> MITENEKISLPKIDWALDALEPYISKEINDLHINKHHVAYVNGYNAAIDALEKAVGKRDLKSVVEIQQ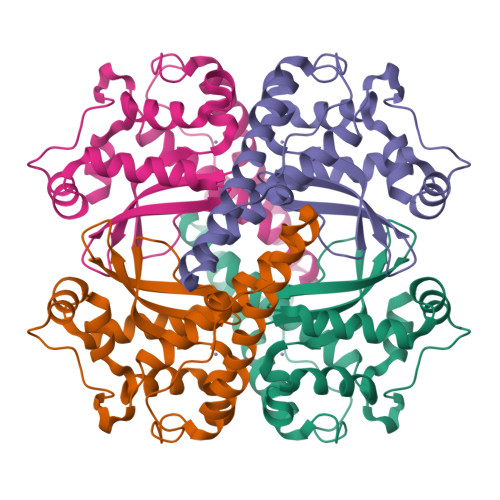NIKFHGGGHTNHSLFWKNLAPVSKGGGKHPDTSSALGKQIVAQYGSVSNLIDITNSKLAGIQGSGWAFIVKNKQNGGALDVVTTANQDTISAPHLVPIIAIDAWEHAYYLQYQNVKLDYFKAIWNVINWAEAESRYSA> SRRVASPSSELRRALEANE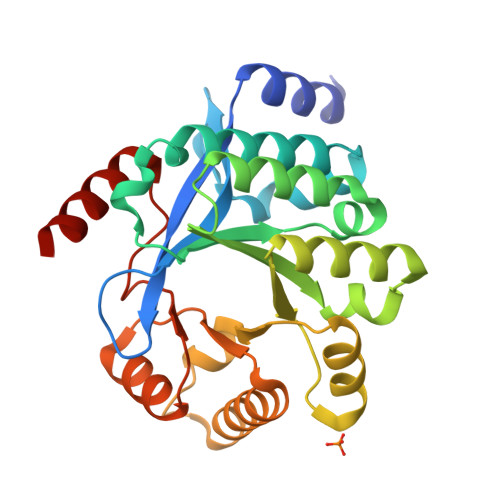FIPYYQPLSPGQGGRWIGVEVLMRWRHPREGLIRPDLFIPFAERSGLIVPMTRALMRQVAEDLGGHAGKLEPGFHIGFNISATHCHELALVDDCRELLAAFPPGHITLVLELTERELIESSEVTDRLFDELHALGVKIAIDDFGTGHSSLAYLRKFQVDCLKIDQSFVARIGIDTLSGHILDSIVELSAKLDLDIVAEGVETPEQRDYLAARGVDYLQGYLIGRPMPLESLLSSLTVQEGQGAS mNeonGreen, an engineered green fluorescent protein (GFP) derived from lancelet, is one of the most brightly fluorescent homologs of Aequorea victoria jellyfish GFP (avGFP) yet reported. However, we were ultimately successful in creating a variant, designated as NeonCyan1, with a tryptophan-derived cyan fluorescent protein (CFP)-type chromophore, and two additional mutants with distinct spectral hues. NeonCyan1 has the ‘double humped’ excitation and emission spectra that are characteristic of FPs with Trp-derived chromophores in the neutral state, such as mTurquoise2 and mCerulean3. To obtain insight into the molecular basis of the empirically determined biophysical and photophysical properties of NeonCyan1 and its variants, we determined the crystal structure of NeonCyan0.95 at close to physiological pH (pH 7.5), NeonCyan0.95 at acidic pH (pH 5.6), and NeonCyan1-T207D at close to physiological pH (pH 6.5).

In addition to obtaining the structure of NeonCyan0.95 at physiological pH, we also obtained the structure of NeonCyan0.95 at an acidic pH (estimated to be ~5.6) which is below the apparent pKa of NeonCyan1 (6.4). The most notable differences between two structures are the different configurations of the chromophore, which is in a Z,Z configuration at physiological pH and Z,E configuration at acidic pH, the presence of a sulfate ion bound in close proximity to the chromophore at acidic pH, and a partial deformation of β-strands 10 and 11. Absorbance spectra of the NeonCyan1 variants in the presence and absence of sulfate ion, at pH 4 and 7.4, did not reveal any substantial effect on the absorption profile. Relative to the Z,Z chromophore stereoisomer in NeonCyan0.95 at pH 7.5, the chromophore of NeonCyan0.95 at pH 5.6 was revealed to be flipped to the Z,E stereoisomer. At acidic pH, the distance to the nitrogen atom of the imidazolinone ring has increased to 3.34 +/− 0.16 Å, which indicates a weaker hydrogen bond and may even be consistent with Glu222 being deprotonated. Associated with this weaker interaction is an outward movement of β-strand 11, which contains Glu220, and β-strand 10. This conformational change may help to sterically accommodate the Z,E stereoisomer of the chromophore. Similarly, the crystal structure of NeonCyan0.95 at pH 5.6 revealed that the chromophore is in the Z,E configuration. This observation supports the conclusion that the NeonCyan1 structure can accommodate the Z,E stereoisomer.

>[8x]MVSKGEEDNMASLPATHELHIFGSINGVDFDMVGQGTGNPNEGYEELNLKSTKGDLQFSPWILVPHVGWGFHQYLPYPDGMSPFQAAMVDGSGYQVHRTMQFEDGASLTVNYRYTYEGSHIKGEAQVKGTGFPADGPVMTNSLTAVDSCWSKKTYPNDKTIISTFKWSYTTGNGERYRSTARTTYTFAKPMAANYLKNQPVYVFRKTELKHSETELNFKEWQKAFTDVMGMDELYK> MKKIVSLLIVAALFCSCSEYQKALKNEDVAAKFEVATKMYDAGKYNKAIRLFEQLAPTYRGKPQAEKLFYMFSQSYYKTKQYYLAGYQFESFVSGYPRSEKVQEAAFLGAYSYSKLAPVYSLDQADTVKALDKLQAFIDNYPNSEYLAQANESVKILNG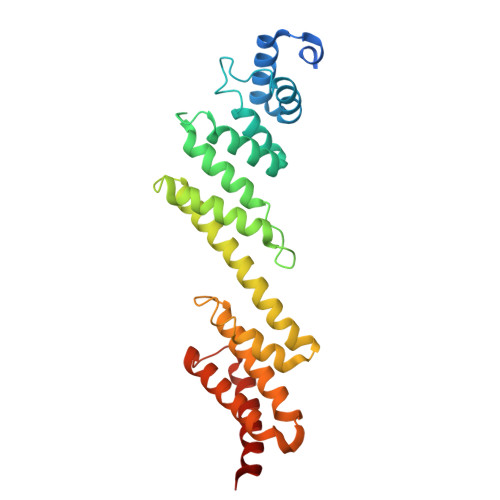KLEKKAYENAKGYNTISDYKSALVAFDNFIADFPGTPLKEDALFYKYDSAYQLAINSVPSKMEERLHVAQTAYANLMKYKSDTKYKEKADQMNARVETDLQKFTK>MLNRVVLVGRLTKDPEYRTTPSGVSVATFTLAVNRTFTNAQGEREADFINCVVFRRQADNVNNYLSKGSLAGVDGRLQSRNYENQEGRRVF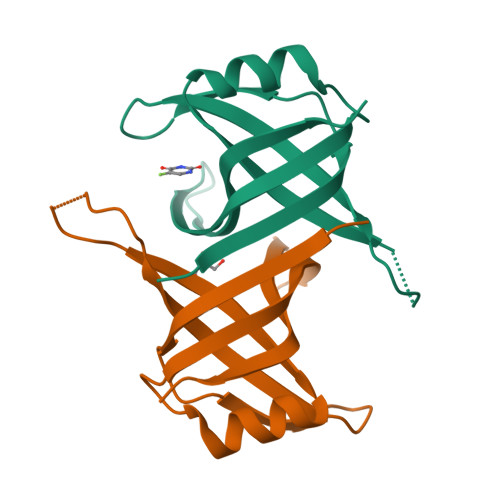VTEVVCDSVQFLEPHHHHHH[2x]>MFTGSIVAIVTPMDEKGNVCRASLKKLIDYHVASGTSAIVSVGTTGESATLNHDEHADVVMMTLDLADGRIPVIAGTGANATAEAISLTQRFNDSGIVGCLTVTPYWNRPSQEGLYQHFKAIAEHTDLPQILYNVPSRTGCDLLPETVGRLAKVKNIIGIKEATGNLTRVNQIKELV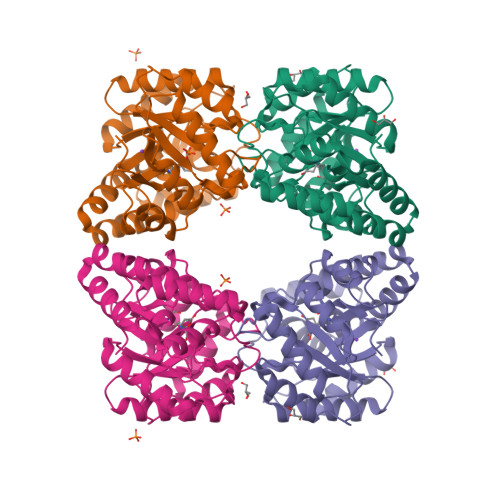SDDFVLLSGDDASALDFMQLGGHGVISVTANVAARDMAQMCKLAAEGHFAEARVINQRLMPLHNKLFVEPNPIPVKWACKELGLVATDTLRLPMTPITDSGRETVRAALKHAGLL[2x]>MVKTRSVNIHVPVKETSKVVLECRGDSYFRHFSYVY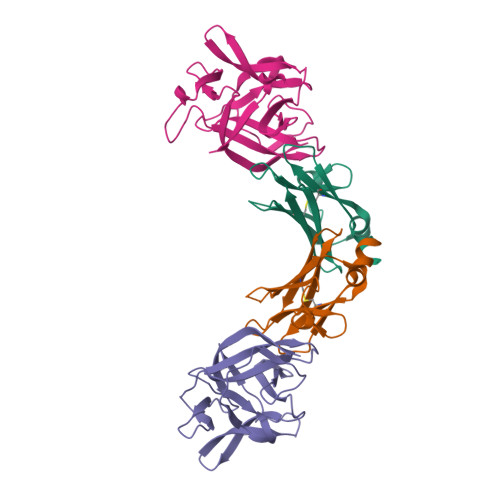WIIGKNKTVDQLPPNSGYRERIYLFKKPHRSENRPRADLILTNITDEMRNEKLTCVLIDPKDPLKESVILSKIWNSVYKI[2x];>[2x]YFGKLESKLSVIRNLNDQVLFIDQGNRPLFEDMTDSDSRDNAPRTIFIISMYKDSQPRGMAVTISVASAAASTLSSENKIISFKEMNPPDNIKDTKSDIIFFQRSVPGHDNKMQFESSSYEGYFLASEKERDLFKLILKKEDELGDRSIMFTVQNED>[3x]ENLMQVYQQARLSNPELRKSAADRDAAFEKINEARSPLLPQLGLGADYTYSNGYRDANGINSNATSASLQLTQSIFDMSKWRALTLQEKAAGIQDVTYQTDQQTLILNTATAYFNVLNAIDVLSYTQAQKEAIY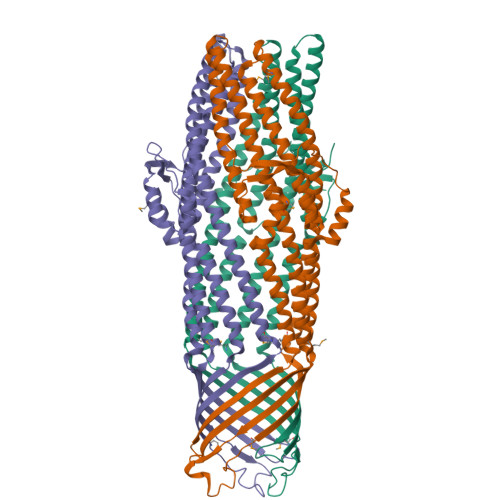RQLDQTTQRFNVGLVAITDVQNARAQYDTVLANELTARNNLDNAVEQLRQITGNYYPELAALNVENFKTDKPQPVNALLKEAEKRNLSLLQARLSQDLAREQIRQAQDGHLPTLDLTASTGISDTSYSGSKTRGAAGTQYDDSNMGQNKVGLSFSLPIYQGGMVNSQVKQAQYNFVGASEQLESAHRSVVQTVRSSFNNINASISSINAYKQAVVSAQSSLDAMEAGYSVGTRTIVDVLDATTTLYNAKQELANARYNYLINQLNIKSALGTLNEQDLLALNNALSKPVSTNPE>MSLDARFDIAHLARAELFSPKPQETLDFFTKFLGMYVTHREGQSVYLRGYEDPYPWSLKITEAPEAG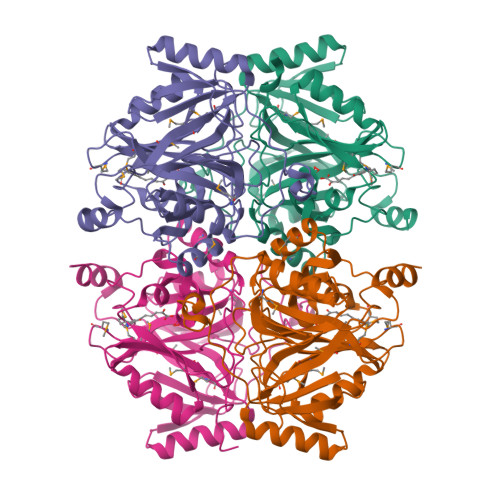MGHAAMRTSSPEALERRAKSLTDGNVDGTWSEDQFGYGKTFEYQSPDGHNLQLLWEAEKYVAPPELRSKILTRPSKKPLQGIPVKRIDHLNLMSSDVTAVKDSFERHLGFRTTERVVDGNVEIGAWMSSNLLGHEVACMRDMTGGHGKLHHLAFFYGTGQHNIDAVEMFRDYDIQIEAGPDKHGITQSQFLYVFEPGGNRIELFGEAGYLHLDPDAETKTWQMSDIDTGLAVGGAKLPWESYFTYGTPSPLSLDQHIEKYAHFGEGHHHHHH[4x]>[2x]SKIFDLVVIGAGSGGLEAAWNAATLYKKRVAVIDVQMVHGPPFFSALGGTCVNVGCVPKKLMVTGAQYMEHLRESAGFGWEFDRTTLRAEWKNLIAVKDEAVLNINKSYDEMFRDTEGLEFFLGWGSLESKNVVNVRESA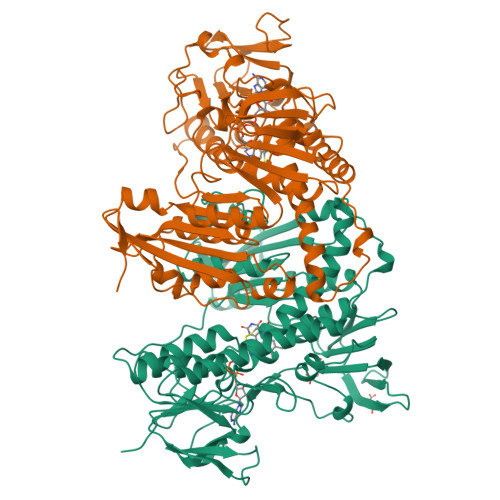DPASAVKERLETEHILLASGSWPHMPNIPGIEHCISSNEAFYLPEPPRRVLTVGGGFISVEFAGIFNAYKPKDGQVTLCYRGEMILRGFDHTLREELTKQLTANGIQILTKENPAKVELNADGSKSVTFESGKKMDFDLVMMAIGRSPRTKDLQLQNAGVMIKNGGVQVDEYSRTNVSNIYAIGDVTNRVMLTPVAINEAAALVDTVFGTTPRKTDHTRVASAVFSIPPIGTCGLIEEVASKRYEVVAVYLSSFTPLMHKVSGSKYKTFVAKIITNHSDGTVLGVHLLGDNAPEIIQGIGICLKLNAKISDFYNTIGVHPTSAEELCSMRTPSYYYVKGEKMEKP>[2x]GPYLQILEQPKQRGFRFRYVCEGPSH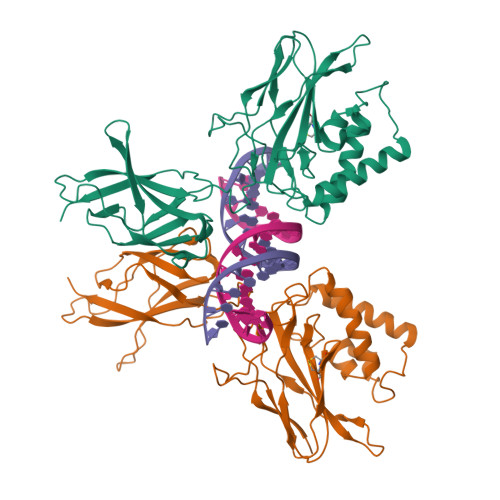GGLPGASSEKNKKSYPQVKICNYVGPAKVIVQLVTNGKNIHLHAHSLVGKHCEDGVCTVTAGPKDMVVGFANLGILHVTKKKVFETLEARMTEACIRGYNPGLLVHSDLAYLQAEGGGDRQLTDREKEIIRQAAVQQTKEMDLSVVRLMFTAFLPDSTGSFTRRLEPVVSDAIYDSKAPNASNLKIVRMDRTAGCVTGGEEIYLLCDKVQKDDIQIRFYEEEENGGVWEGFGDFSPTDVHRQFAIVFKTPKYKDVNITKPASVFVQLRRKSDLETSEPKPFLYYPE>[2x]ASELNIYSARHYNADFEIIKKFEEKTGIKVNHTQAKASELIKRLSLEGSNSPADIFITADISNLTEAKNLGLLSPVSSKYLEEFIPAHLRDKDKEWFAITKRARIIAYNKNTNIDISKMKNYEDLAKAEFKGEIVMRSATAPYSKTLLASIIANDGNKEAKAWAKGVL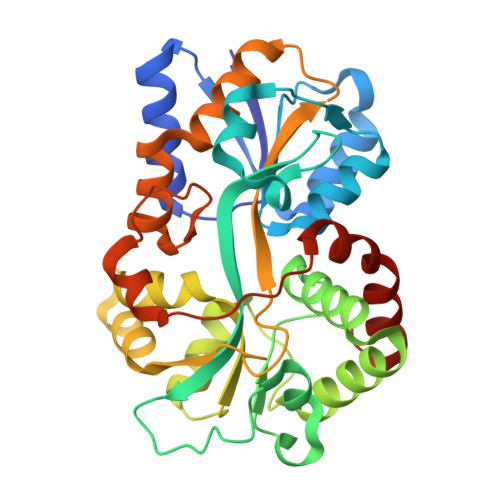ENLATNPKGGDRDQARQVFAGEAKFAVMNTYYIGLLKNSKNPKDVEVGNSLGIIFPNQDNRGTHINISGIAMTKSSKNQDAAKKFMEFMLSPEIQKILTDSNYEFPIRNDVELSQTVKDFGTFKEDQIPVSKIAENIKEAVKIYDEVGFRIEGR>[2x]GSPCPGACVCYNEPKVTT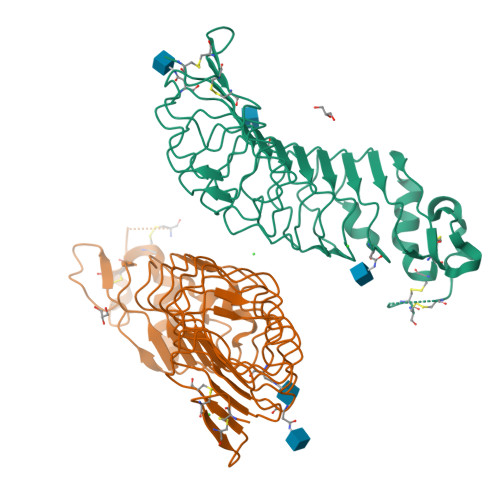SCPQQGLQAVPTGIPASSQRIFLHGNRISHVPAASFQSCRNLTILWLHSNALARIDAAAFTGLTLLEQLDLSDNAQLHVVDPTTFHGLGHLHTLHLDRCGLRELGPGLFRGLAALQYLYLQDNNLQALPDNTFRDLGNLTHLFLHGNRIPSVPEHAFRGLHSLDRLLLHQNHVARVHPHAFRDLGRLMTLYLFANNLSMLPAEVLMPLRSLQYLRLNDNPWVCDCRARPLWAWLQKFRGSSSEVPCNLPQRLADRDLKRLAASDLEGCAVASGPFRPIQTSQLTDEELLSLPKCCQPDAADKASVLEAAAHHHHHH>[2x]AAASFGQTKIPRGNGPYSVGCTDLMFDHTNKGTFLRLYYPSQDNDRLDTLWIPNKEYFWGLSKF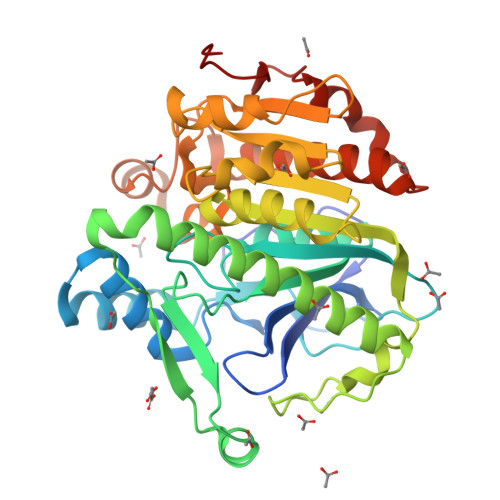LGTHWLMGNILRLLFGSMTTPANWNSPLRPGEKYPLVVFSHGLGAFRTLYSAIGIDLASHGFIVAAVEHRDRSASATYYFKDQSAAEIGDKSWLYLRTLKQEEETHIRNEQVRQRAKECSQALSLILDIDHGKPVKNALDLKFDMEQLKDSIDREKIAVIGHSFGGATVIQTLSEDQRFRCGIALDAWMFPLGDEVYSRIPQPLFFINSEYFQYPANIIKMKKCYSPDKERKMITIRGSVHQNFADFTFATGKIIGHMLKLKGDIDSNVAIDLSNKASLAFLQKHLGLHKDFDQWDCLIEGDDENLIPGTNINTTNQHI> DTAWERYKARFMMPDGRIIDTANGNVSHTEGQGFAMLLAVANNDRPAFDKLWQWTDSTLRDKSNGLFYWRYNPVAPDPIADKNNASDGDTLIAWALLRAQKQWQDKRYAIASDAITASLLKYTVVTFAGRQVMLPGVKGFNLNDHLNLNPSYFIFPAWRAFAERTHLTAWRTLQTDGQALLGQMGWGKSHLPSDWVALRADGKMLPAKEWPPRMSFDAIRIPLYLSWADPQSALLAPWKAWMQ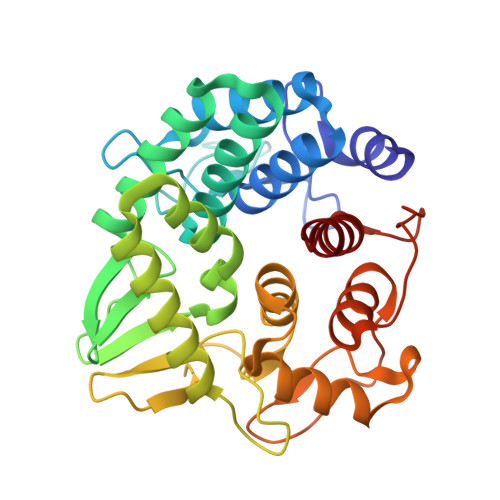SYPRLQTPAWINVSTNEVAPWYMAGGLLAVRDLTLGEPQEAPQIDDKDDYYSASLKQLVWLAKQDQR> IVGGTNSSWGEWPWQVSLQVKLTAQRHLCGGSLIGHQWVLT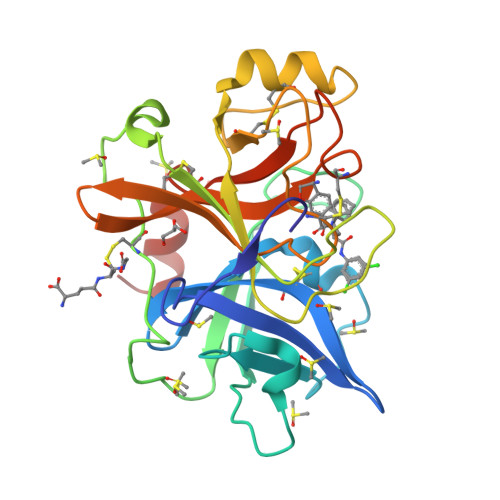AAHCFDGLPLQDVWRIYSGILNLSDITKDTPFSQIKEIIIHQNYKVSEGNHDIALIKLQAPLNYTEFQKPICLPSKGDTSTIYTNCWVTGWGFSKEKGEIQNILQKVNIPLVTNEECQKRYQDYKITQRMVCAGYKEGGKDACKGDSGGPLVCKHNGMWRLVGITSWGEGCARREQPGVYTKVAEYMDWILEKTQSSDGKA> IDPRFPHHHPRPQSFWEARAKALESLLIEKGHLSSDASERVIKHYEHELGPMNGAKVVAKAWTDPAFKQRLLEDSETVLRELGYYGLQGEHIRVVENTDTV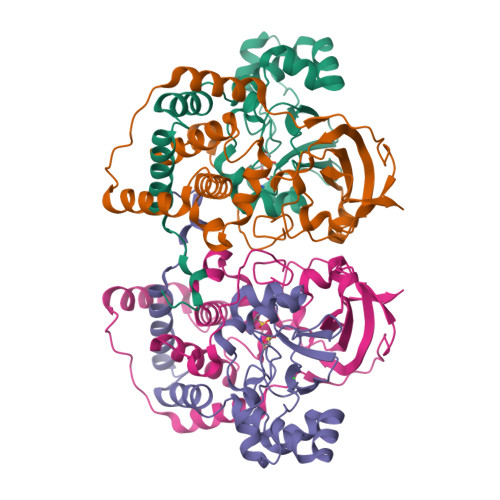HNVVVCTLCSCYPWPLLGLPPSWYKEPAYRARVVKEPRQVLKEFGLDLPDSVEIRVWDSSSEIRFMVLPQRPEGTEGMTEEELAKLVTRDSMIGVAKIEPPKVTVG;> MNGIHDVGGMDGFGKVMYVKEEEDIYFTHDWERLAFGLVAGCMAQGLGMKAFDEFRIGIELMRPVDYLTSSYYGHWIATVAYNLVDTGVLDEKELDERTEVFLKKPDTKIPRREDPALVKLVEKALYDGLSPLREISASPRFKVGERIKTKNIHPTGHTRFPRYARDKYGVIDEVYGAHVFPDDAAHRKGENPQYLYRVRFEAEELWGYKQKDSVYIDLWESYMEPVSH> MMRISRKLLVPVANFRPKKPWDGPWGIQISQKKDRPFIAMWILFPLLLVDHLTR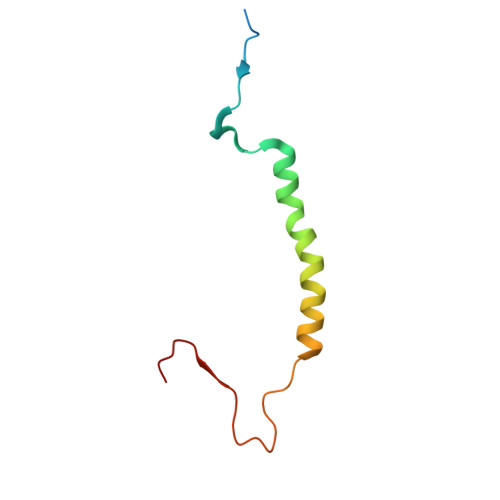EYYAYWHSSKVPVTDVFGDF>[2x]NAVTEEQLTFSQAMGDMLATWQLPRTTGRTYGYLLLQSEAT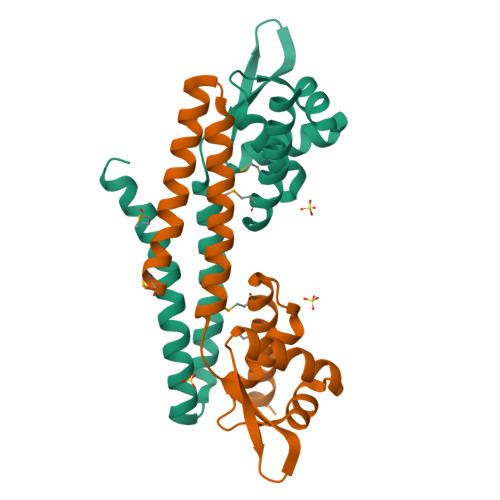SFQEIGADLGLSPGAVSTSVRELVAWGLARTIPQPGSRRLLVEAAGGFEQLLAASHERSRAFIRTLRSGQALADDDRVATRLVDLTDLFEAYVEAGEQMLRRRHEAGG> MKRLFPSAGVSVVLTSSSIVMSCPCNHIFTSRRAYYWPYNEDFVPEGAETSRFQSSGSPGTRRRVLQEYALSPLFGARVPCCVVGTLRTAKEIIVLKRDIQSLLCELMELPQGSVT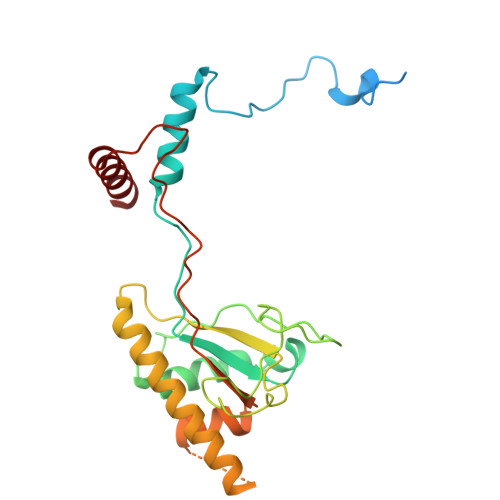LGPLQQLREMMLYRHGTPLSPRLGDERQLNMDAYARRPIAARTMMDVFLAEDMSLDEIVNFGRLSLGKLQIALNNLRKENAEKSSADCEDGSAVEPAQLLVDRMGISYCEIPSLDESDYVFAEVGGVAVTDEEAERVAQRWAERCE>SYYHHHHHHLESTSLYKKAGLRILAIDTATEACSVALWNDGTVNAHFELCPREHTQRILPMVQDILTTSGTSLTDINALAYGRGPGSFTGVRIGIGIAQGLALGAELPMIGVSTLMTMAQGAWRKNGATRVLAAIDARMGEVYWAEYQRDENGIWHGEETEAVLKPEIVHERMQQLSGEWVTVGTGWQAWPDLGKESGLVLR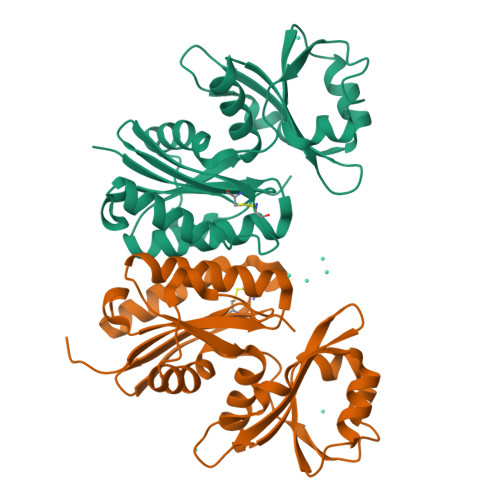DGEVLLPAAEDMLPIACQMFAEGKTVAVEHAEPVYLRNNVAWKKLPGKE[4x]> ENLYFQSNAMRLPYSWLREVVAVGASGWDVTPGELEQTLLRIGHEVEEVIPLGPVDGPVTVGRVADIEELTGYKKPIRACAVDIGDRQYREIICGATNFAVGDLVVVALPGATLPGGFTISARKAYGRNSDGMICSAAELNLGADHSGILVLPPGAAEPGADGAGVLGLDDVVFHLAITPDRGYCMSVRGLARELACAYDLDFVD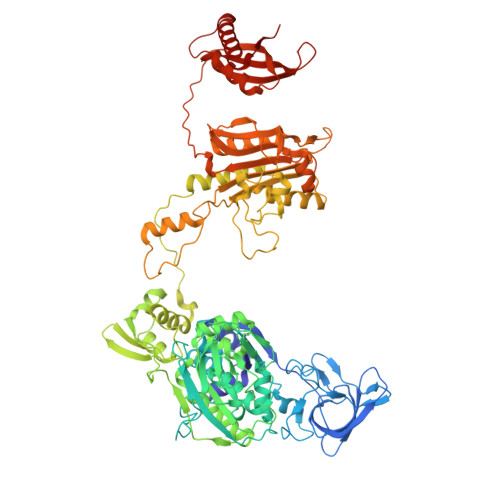PASNSRVPPLPIEGPAWPLTVQPETGVRRFALRPVIGIDPAAVSPWWLQRRLLLCGIRATCPAVDVTNYVMLELGHPMHAHDRNRISGTLGVRFARSGETAVTLDGIERKLDTADVLIVDDAATAAIGGVMGAASTEVRADSTDVLLEAAIWDPAAVSRTQRRLHLPSEAARRYERTVDPAISVAALDRCARLLADIAGGEVSPTLTDWRGDPPCDDWSPPPIRMGVDVPDRIAGVAYPQGTTARRLAQIGAVVTHDGDTLTVTPPSWRPDLRQPADLVEEVLRLEGLEVIPSVLPPAPAGRGLTAGQQRRRTIGRSLALSGYVEILPTPFLPAGVFDLWGLEADDSRRMTTRVLNPLEADRPQLATTLLPALLEALVRNVSRGLVDVALFAIAQVVQPTEQTRGVGLIPVDRRPTDDEIAMLDASLPRQPQHVAAVLAGLREPRGPWGPGRPVEAADAFEAVRIIARASRVDVTLRPAQYLPWHPGRCAQVFVGESSVGHAGQLHPAVIERSGLPKGTCAVELNLDAIPCSAPLPAPRVSPYPAVFQDVSLVVAADIPAQAVADAVRAGAGDLLEDIALFDVFTGPQIGEHRKSLTFALRFRAPDRTLTEDDASAARDAAVQSAAERVGAVLRG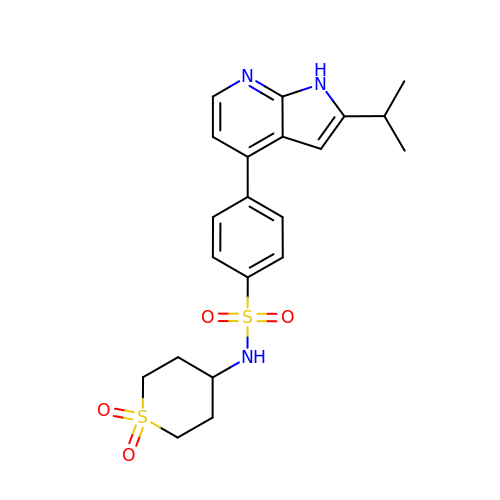N-(1,1-dioxidotetrahydro-2H-thiopyran-4-yl)-4-[2-(1-methylethyl)-1H-pyrrolo[2,3-b]pyridin-4-yl]benzenesulfonamide | C21 H25 N3 O4 S2 | QBYYCHRRPPTEBG-UHFFFAOYSA-N Apolipoprotein C-1 (APOC1) is a 57 amino acid polypeptide of Mr = 6.6 kDa that is synthesized predominantly in the liver of mammals. In humans, the plasma concentration is about 6 mg/dl. This small protein is remarkable for being the most positively charged protein in the human body, with a lysine content of 17%. The protein has a high affinity for lipid surfaces, particularly chylomicrons, and both HDL and VLDL particles. APOC1 had long been known to be a crucial player in the transfer of lipids between particles and the general clearance of lipids, but its mechanism and the manner by which it bound to lipoprotein particles was poorly understood. It was then discovered that APOC1 is a potent inhibitor of cholesteryl ester transferase protein (CETP), which is the crucial enzyme in the transfer of cholesterol between lipid surfaces (tissues) and lipid particles.

The structure consists of two basically identical long α-helices, closely associated with one another and aligned in an antiparallel fashion. The helices are about 75 Å long and have 13–14 helical turns. The structure is clearly a natural dimer; it is not a consequence of crystal packing. The total buried surface area on the two monomers comprising the dimer is 2,595 Å2, or about 15% of the total surface area (18,355 Å2) of the dimer (program PISA; CCP4). On one monomer (A), on the amino-terminal half, there is a near-continuous stack of hydrophobic side chains. These are Leu11-Phe14-Leu18-gap-Leu25-Ileu29, with a gap between Leu18 and Leu25. On the other monomer, closely opposed to the stack on monomer A, is a different stack of hydrophobic side chains from the carboxy-terminal half of molecule B. This stack is Leu53-Val49-Phe46-Trp41-Phe42-Met38-Leu34. The two opposing hydrophobic stacks are not only in direct contact, but are further consolidated by the intercalation of part of the side chain of Trp41 into the gap of the opposite stack between Leu18 and Leu25. In the less hydrated (34% solvent) Monocl-1 crystals, and the even less hydrated (25% solvent) Monocl-2 crystals, dimers are so closely packed, molecule A against B of translationally related dimers, that the sheet or band is extremely dense.

>MRLFLSLPVLVVVLSIVLEGPAPAQGTPDVSSALDKLKEFGNTLEDKARELISRIKQSELSAKMREWFSETFQKVKEKLKIDS[2x]>MANPTLFVSYDQNGKKLSFANWISVLSPQDTPFVSMTGKESINQTIFSWQTDALASVDGNNAHVEGSRAEDGEMKPTVIKSNVTQILRKVVRVSDTANTTANY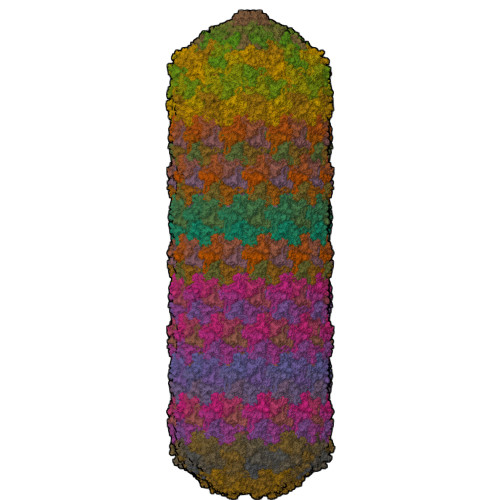GRGRELMYQLEKKGKEIKRDLEKILLSGQARTDVLADQYLTNSAADPAVAGLNDTHAARKTGAFQFLCAHGGLAGGVVDKTKNGPADPDTGAVTVKVAQNASNPTTNIGFDEADIFDMTLQLYTAGSEADIIMINPAHAKIFAGLQENTQGSRKRIFENTKQFIYEVNSITDPLGQSYKIIVNRWMPTDAVYFFRSADWTQMVLRAPKRTELAKDGSYEKWMIEMEVGLRHRNPYASGVLFTAAGKAAA[95x]>GMLEGLEAVRKRPGMYIGSTGERGLHHLIWEVVDNAVDEAMAGHATKVRVRLLADGGVEVSDDGRGIPVEMHESGVPTVDVVMTQVGVSVVNALSTRMEVEICRDGYQWFQTYDKSVPGTLKQGEKTRKTGTVVRFWPDPDVFETTTFDFETVARRLQEQAFLNKGLTIELIDERDGKHRTFYYPG[2x]

Gyrase is a type II topoisomerase and the only enzyme that can catalyse the introduction of negative supercoils into DNA;3,5 it is composed of two subunits, GyrA and GyrB, which form an A2B2 complex in the active enzyme. Gyrase is an essential enzyme in bacteria and has been extensively studied as a target for antibacterial agents;6 gyrase has been described as an effective drug target for the development of new anti-TB agents. Other compounds, such as the aminocoumarins (e.g. novobiocin), inhibit gyrase through targeting the ATPase domains of gyrase and topo IV, located in the N-terminal domain of GyrB (and ParE), thus preventing supercoiling. In addition, we present crystal structures of the GyrB N-terminal ATPase sub-domain from Mycobacterium thermoresistibile bound to one of these compounds (Redx03863) and also to novobiocin, demonstrating that this novel compound class inhibits via a binding pocket and resistance mechanism different from that of novobiocin.

We have investigated gyrase from M. thermoresistibile and found it to be more stable than the M. tuberculosis enzyme. Based on these findings, we successfully co-crystallized a 21 kDa N-terminal sub-domain of M. thermoresistibile GyrB (residues 20–254 with residues 103–122 and 214–244 excluded) with novobiocin and Redx03863. This N-terminal sub-domain had been previously used to determine the novobiocin-binding site in gyrase from other organisms. Superposition of the two mycobacterial novobiocin complexes gave a root mean square deviation (RMSD) value of 0.688 Å, indicating that they are closely similar. Residue Arg141 (Arg136 in E. coli) makes a key contact to the aminocoumarin ring system of novobiocin;39–41 the direct interaction between Arg141 and the aminocoumarin ring system of novobiocin has been crystallographically confirmed, and mutation at this residue leads to resistance to the drug.> MGKTKTRGRRHQDKQRKDEFEPSSNSAKEHIQQEESTYNDEAEIKETQPQMFFGVLDREELE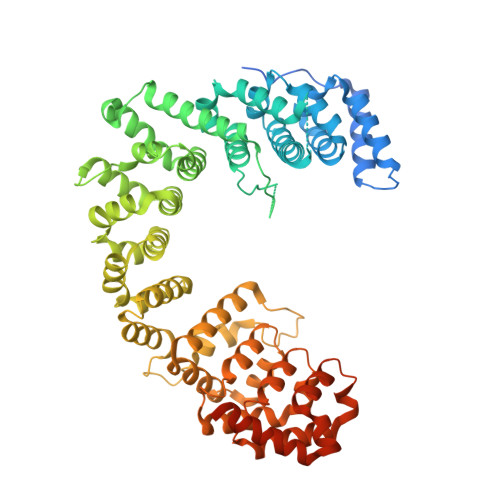YFKQAESTLQLDAFEAPEEKFQFVTSIIEEAKGKELKLVTSQITSKLMERVILECDETQLKDIFQSFNGVFFGLSCHKYASHVLETLFVRSAALVERELLTPSFDNNEKEGPYVTMENMFLFMLNELKPHLKTMMNHQYASHVLRLLILILSSKTLPNSTKANSTLRSKKSKIARKMIDIKDNDDFNKVYQTPESFKSELRDIITTLYKGFTNGAESRSDISQSTITKFREYSVDKVASPVIQLIIQVEGIFDRDRSFWRLVFNTADEKDPKEESFLEYLLSDPVGSHFLENVIGSARLKYVERLYRLYMKDRIVKLAKRDTTGAFVVRALLEHLKEKDVKQILDAVVPELSMLLNSNMDFGTAIINASNKQGGYLRDDVIAQLIQKYYPEKSDAKNILESCLLLSASTLGNTRDDWPTAEERRRSVFLEQLIDYDDKFLNITIDSMLALPEERLIQMCYHGVFSHVVEHVLQTTRVDIIKRKMLLNILSKESVNLACNVYGSHIMDKLWEFTAKLTLYKERIARALVLETEKVKNSIYGRQVWKNWKLELYVRKMWDWKKLIKEQEFEIFPNSKPLQPKPEKHSRERNNSKEGSAFKKQKHYR2-(2,4-difluorophenyl)-N-(pyridin-3-yl)acetamide | C13 H10 F2 N2 O | 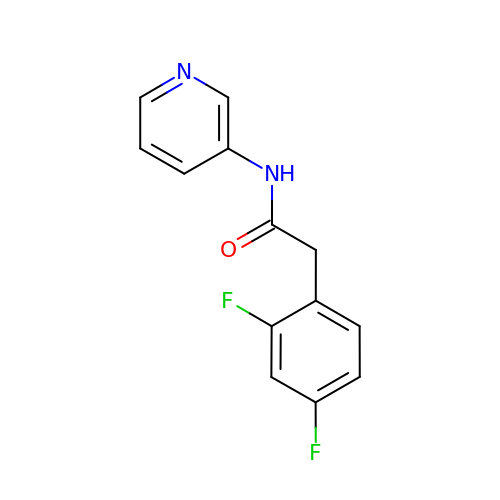RWAUIOABZSEIGJ-UHFFFAOYSA-N> MSEKWKE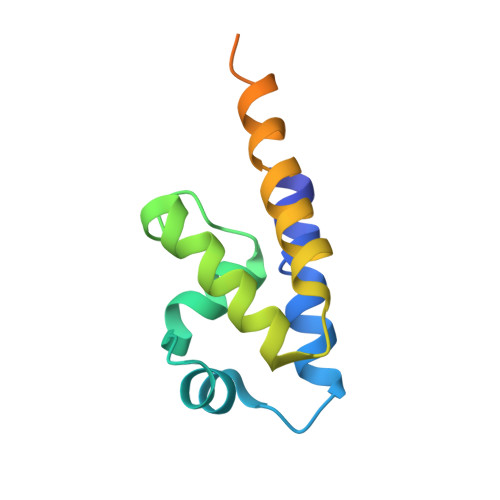LGETFRKKREERRITLLDASLFTNINPSKLKRIEEGDLKGLDAEVYIKSYIKRYSEFLELSPDEMLKLYEEGKEEVAEEVEEKKPRKKKEKEKTRDLGSHHHHHH(7-methyl-2,3-dihydroindol-1-yl)-(1,2,3-triazol-1-yl)methanone 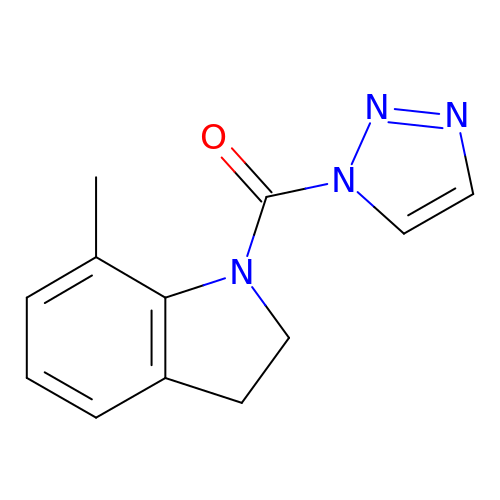| C12 H12 N4 O | SKGYNFOODZJUGQ-UHFFFAOYSA-N>MSDKLPYKVADIGLAAWGRKALDIAENEMPGLMRMREMYSASKPLKGARIAGCLHMTVETAVLIETLVALGAEVRWSSCNIFSTQDHAAAAIAKAGIPVFAWKGETDEEYLWCIEQTLHFKDGPLNMILDDGGDLTNLIHTKYPQLLSGIRGISEETTTGVHNLYKMMSNGILKVPAINVNDSVTKSKFDNLYGCRESLIDGIKRATDVMIAGKVAVVAGYGDVGKGCAQALRGFGARVIITEIDPINALQAAMEGYEVTTMDEACKEGNIFVTTTGCVDIILGRHFEQMKDDAIVCNIGHFDVEIDVKWLNENAVEKVNIKPQVDRYWLKNGRRIILLAEGRLVNLGCAMGHPSFVMSNSFTNQVMAQIELWTHPDKYPVGVHFLPKKLDEAVAEAHLGKLNVKLTKLTEKQAQYLG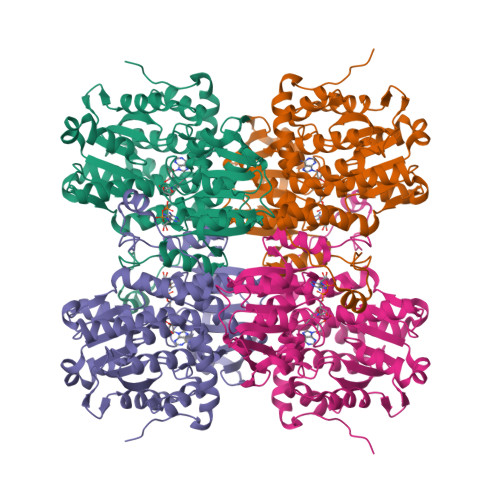MPINGPFKPDHYRY[2x]>EAPHLVQVDAARALWPLRRFWRSTGFCPPLPHSQADPYVLSWDQQLNLAYVGAVPHRGIKQVRTHWLLELVTTRGSTGQGLSYNFTHLDGYLDLLRENQLLPGFELMGSASGHFTDFEDKQQVFEWKDLVSSLARRYIGRYGLAHVSKWNFETWNEPDHHDFDNVSMTMQGFLNYYDACSEGLRAASPALRLGGPGDSFHTPPRSPLSWGLLRHCHDGTNFFTGEAGVRLDYISLHRKGARSSISILEQEKVVAQQIRQLFPKFADTPIYNDEADPLVGWSLPQPWRADVTYAAMVVKVIAQHQNLLLANTTSAFPYALLSNDNAFLSYHPHPFAQRTLTARFQVNNTRPPHVQLLRKPVLTAMGLLALLDEEQLWAEVSQAGTVLDSNHTVGVLASAHRPQGPADAWRAAVLIYASDDTRAHPNRSVAVTLRLRGVPPGPGLVYVTRYLDNGLCSPDGEWRRLGRPVFPTAEQFRRMRAAEDPVAAAPRPLPAGGRLTLRPALRLPSLLLVHVCARPEKPPGQVTRLRALPLTQGQLVLVWSDEHVGSKCLWTYEIQFSQDGKAYTPVSRKPSTFNLFVFSPDTGAVSGSYRVRALDYWARPGPFSDPVPYLEVPVPRGPPSPGNP[2x]

Human α‐l‐iduronidase (IDUA), which belongs to the GH39 family in the Carbohydrate Active EnZyme (CAZy) classification, hydrolyzes terminal non‐reducing α‐l‐iduronic acid residues in glycoaminoglycans (GAGs), including dermatan sulfate (DS) and heparan sulfate (HS), through a two‐step Koshland double‐displacement mechanism. The active site of the enzyme contains a carboxylic acid/carboxylate pair that acts as an acid/base (Glu188) and a nucleophilic (Glu299) catalyst. Mutations in the gene encoding IDUA may result in mucopolysaccharidosis type I (MPS I), which is a rare autosomal inherited recessive disease that leads to toxic accumulation of HS and DS. The structures of IDUA when complexed with the inhibitors in a non‐covalent transition state mimicking form and a covalent enzyme‐bound form provide insights into its conformational itinerary.

Data were collected from a crystal soaked with ABP 1 for 24 h to 2.02 Å resolution, which revealed the structure of raIDUA in a covalent complex with 1. The aziridine nitrogen is displaced by nucleophilic attack of the active site carboxylate to form a trans‐2‐amino ester (with the rest of the R group not visible in the electron density, presumably disordered due to its inherent flexibility; this region of the structure is exposed to the solvent). Interestingly, the pseudo‐glycoside was observed in a 5S1 skew‐boat conformation, which differs slightly from the distorted 2, 5B boat conformation reported for the previously described irreversible inhibitor 2‐deoxy‐2‐fluoro‐α‐l‐ido‐pyranosyl uronic acid (2F‐IdoA) covalently bound to IDUA. The observed 5S1 conformation of the covalent inhibitor 1–enzyme complex supports predictions for the conformational itinerary followed by α‐iduronidase GH39. The carboxylate group of the pseudo‐iduronic acid forms bidentate hydrogen bonds with the main‐chain nitrogen atoms of Gly305 and Trp306, the C4 hydroxyl group forms hydrogen bonds with Arg363 and Asp349, the C3 hydroxyl group interacts with Asp349 and a water molecule, and the C2 hydroxyl group forms hydrogen bonds with Asn181 and the nucleophile Glu299. In the covalent complex between IDUA and 2F‐IdoA, the nucleophile Glu299 is rotated by around 90° compared to the position observed in the complex here with the fragment of 1,8 and the fluoro group at C2 may preclude an interaction with Oϵ2 of Glu299, causing it to rotate. However, the inhibitor 1–IDUA complex presented here, bearing a hydroxyl group at C2 and showing an interaction with Glu299, is more likely to represent what occurs during catalysis. Superimposition of the main‐chain atoms for the two complexes revealed a shift in the position of the cyclophellitol aziridine to accommodate formation of the covalent bond. This engendered movement of between 0.2 and 0.4 Å at C5, C4, and C3, 0.5 Å at C2, 0.6 Å at the carbon at the position of the endocyclic oxygen, and 1.1 Å at the pseudo‐anomeric carbon.>[2x]MYGLVNKAIQDMISKHHGEDTWEAIKQKAGLEDIDFFVGMEAYSDDVTYHLVGAASEVLGKPA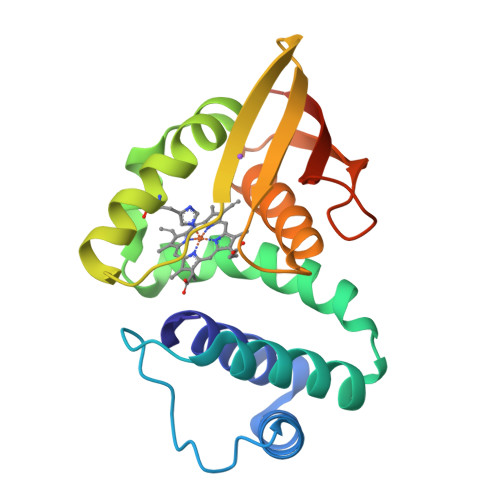EELLIAFGEYWVTYTSEEGYGELLASAGDSLPEFMENLDNLHARVGLSFPQLRPPAFECQHTSSKSMELHYQSTRCGLAPMVLGLLHGLGKRFQTKVEVTQTAFRETGEDHDIFSIKYEDSNLYDD> MGHHHHHHSHMDVAPLNLGMIAAYYYINYTTIELFSMSLNAKTKVRGLIEIISNAAEYENIPIRHHEDNLLRQLAQKVPHKLNNPKFNDPHVKTNLLLQAHLSRMQLSAELQSDTEEILSKAIRLIQACVDVLSSNGWLSPALAAMELAQMVTQAMWSK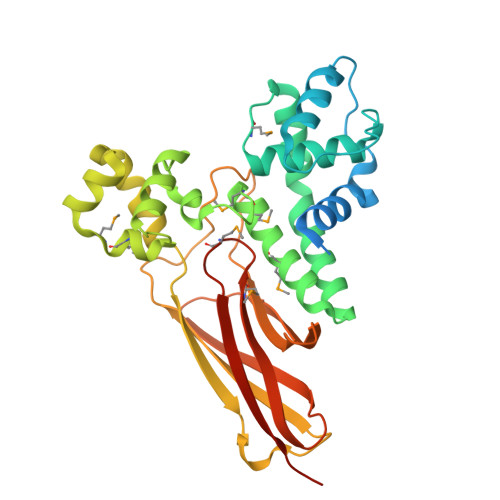DSYLKQLPHFTSEHIKRCTDKGVESVFDIMEMEDEERNALLQLTDSQIADVARFCNRYPNIELSYEVVDKDSIRSGGPVVVLVQLEREEEVTGPVIAPLFPQKREEGWWVVIGDAKSNSLISIKRLTLQQKAKVKLDFVAPATGAHNYTLYFMSDAYMGCDQEYKFSVDVKEAETDSDSD~{N}-[3-(1,3-benzodioxol-5-yl)pyrazolo[1,5-a]pyrimidin-5-yl]-~{N}',~{N}'-dimethyl-propane-1,3-diamine 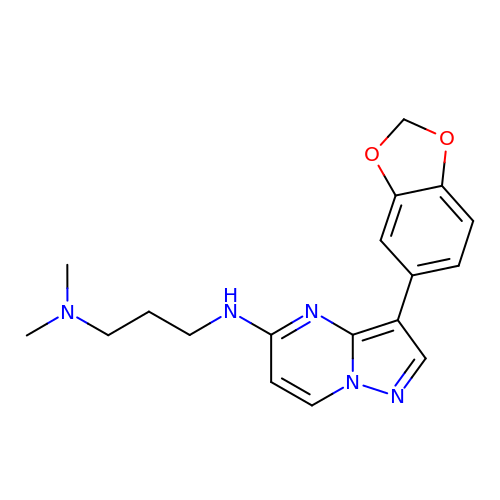| C18 H21 N5 O2 | DQYRQFLRDJTHQM-UHFFFAOYSA-N>MITSSLPLTDLHRHLDGNIRTQTILELGQKFGVKLPANTLQTLTPYVQIVEAEPSLVAFLSKLDWGVAVLGDLDACRRVAYENVEDALNARIDYAELRFSPYYMAMKHSLPVTGVVEAVVDGVRAGVRDFGIQANLIGIMSRTFGTDACQQELDAILSQKNHIVAVDLAGDELGQPGDRFIQHFKQVRDAGLHVTVHAGEAAGPESMWQAIRDLGATRIGHGVKAIHDPKLMDYLAQHRIGIESCLTSNLQTSTVDSLATHPLKRFLEHGILACINTDDPAVEGIELPYEYEVAAPQAGLSQE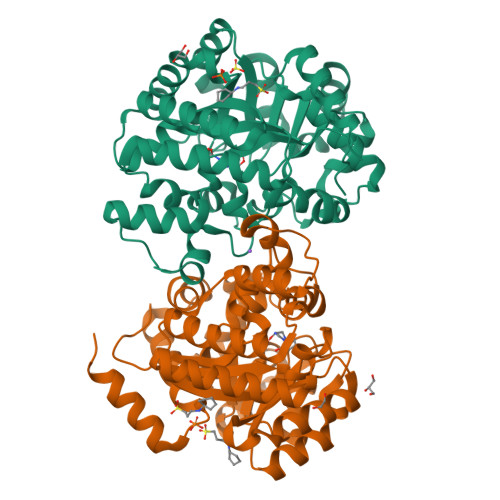QIRQAQLNGLELAFLSDSEKKALLAKAALRGHHHHHH[2x]> MEIVYKPLDIRNEEQFASIKKLIDADLSEPYSIYVYRYFLNQWPELTYIAVDNKSGTPNIPIGCIVCKMDPHRNVRLRGYIGMLAVESTYRGHGIAKKLVEIAIDKMQREHCDEIMLETEVENSAALNLYEGMGFIRMKRMFRYYLNEGDAFKLILPLT;> GPMEVDSILGSLSITDDFDQLVDVTSLFDELCSKLKPEAIVKDPRFDLFEGTHSLEVNNSKLDSSLIELTAEEIEFDVNVAYDPPLASVAAIADRLLRCVISWLNDYQTLPTTVLSCRYTESLLSSLVKGTTAGSSWCTGNILYDKVLGSCILGVCYLTKFVQKLLSAGIVFEEEDLNFNNMGFNTFDNLPGQDVVINSLTESLQILEAYSDDSLHLTMLKHILKIIICLVHLEDHLTDYSTKTSHLDELIENANSVNGIFPQLQLSPPKGAFSTYIQKHRSNQFPPRKITKLPTDYSGFITLANDVKTILLVDKAESALETYQFAKFFNKLEQRHVIARILFPLFFIRDDRTVLGKFSYTQFYLLHVKEFSAQTPSEFESSIGNELIQESSNMLLEWYQNCSQNTCRYRQGFNRQLILWDSLQAQFESVNSQVYCSWTYFMKLSSMIEFSLKGFDLDIYKPFEAYSMFWYVYYLSHHLETFLKDSQNDIESNINAIHSMNKKLKKLKAGEKKDQLRLKYRFAMDNEMEQLQATKQFLNYLLKEINITKSLCLIEVFQFAILKSFGLIDNKNSTPSKFSNERLIHNLRFKPFNSIGVPELPEYEVFQQTLKDFVIEEKGAAFDIKLERATNFIETEVRNVVSSIDEIMQGIKGGDNNGVLVTGTRLVQELSLEY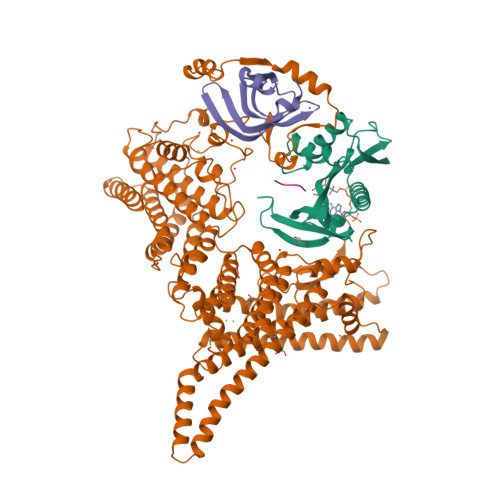YCKLKHTSKALSVNSKVIVNTLKKNIKNKDSHEYKVELVHTTEGWNYFPIQTLRIKQDRYK;> MDILKLSDFIGNTLIVSLTEDRILVGSLVAVDAQMNLLLDHVEERMGSSSRMMGLVSVPRRSVKTIMIDKPVLQELT;> MFHLVGSRRR> SMIRKQAESYANSTWEVLQYKDSGEPGVLEVFVTINGKVQNITFHIPKTIYMKFKSQTMPLQKIKNCLIEKSSASLPNNPKTSNPAGGQLFKITLPESVFLEEKENCTSIFNDENVLGVFEGTITPHQRAIMDLGASVTFRSKAMGALGKGIQQGFEMKDLSMAENERYLSGFSMDIGYLLHFPTSIGYEFFSLFKSWGDTITILVLKPSNQAQEINASSLGQIYKQMFEKKKGKIETYSYLVDIKEDINFEFVYFTDISKLYRRLSQETTKLKEERGLQFLLLLQSPFITKLLGTIRLLNQMPIVKLSLNEVLLPQLNWQPTLLKKLVNHVLSSGSWISHLIKLSQYSNIPICNLRLDSMDYIIDVLYARKLKKENIVLWWNEKAPLPDHGGIQNDFDLNTSWIMNDSEFPKINNSGVYDNVVLDVGVD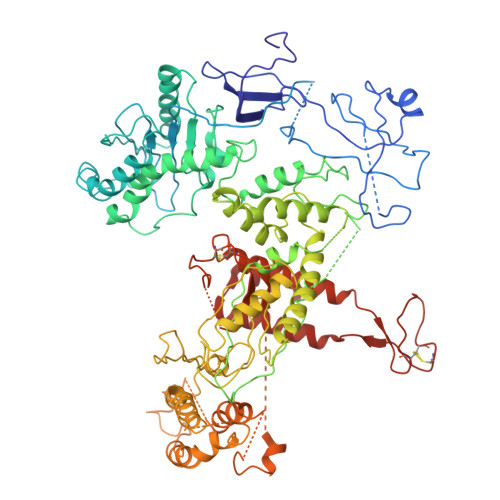NLTVNTILTSALINDAEGSDLVNNNMGIDDKDAVINSPSEFVHDAFSNDALNVLRGMLKEWWDEALKENSTADLLVNSLASWVQNPNAKLFDGLLRYHVHNLTKKALLQLVNEFSALGSTIVYADRNQILIKTNKYSPENCYAYSQYMMKAVRTNPMFSYLDLNIKRYWDLLIWMDKFNFSGLACIEIEEKENQDYTAVSQWQLKKFLSPIYQPEFEDWMMIILDSMLKTKQSYLKLNSGTQRPTQIVNVKKQDKEDSVENSLNGFSHLFSKPLMKRVKKLFKNQQEFILDPQYEADYVIPVLPGSHLNVKNPLLELVKSLCHVMLLSKSTILEIRTLRKELLKIFELREFAKVAEFKDPSLSLVVPDFLCEYCFFISDIDFCKAAPESIFSCVRCHKAFNQVLLQEHLIQKLRSDIESYLIQDLRCSRCHKVKRDYMSAHCPCAGAWEGTLPRESIVQKLNVFKQVAKYYGFDILLSCIADLT N-(cyclopropylmethyl)-2,2,3,3-tetramethylazetidine-1-carboxamide 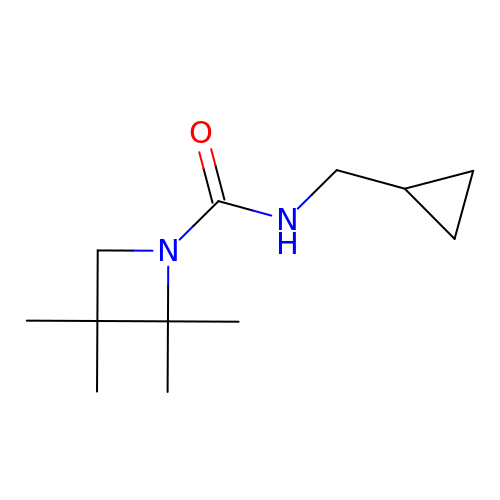| C12 H22 N2 O | SMWGIHJAGGUFFL-UHFFFAOYSA-N> GSHMIWEQHTVTLHRAPGFGFGIAISGGRDNPHFQSGETSIVISDVLKGGPAEGQLQENDRVAMVNGVSMDNVEHAFAVQQLRKSGKNAKI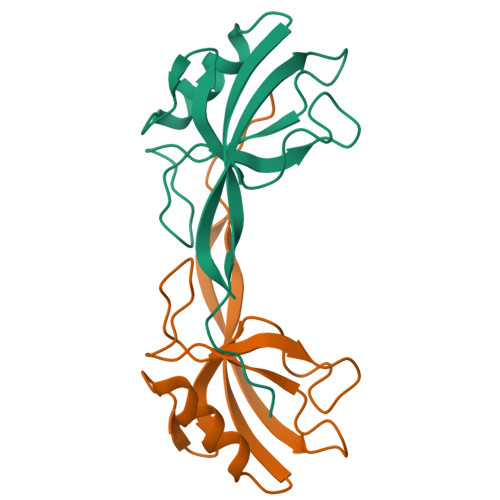TIRRKKGGGWRRTTWV> MSEVFLELGQRPDEAGPPISGPATYPDDVTESLRADAEQIIARYPDARSA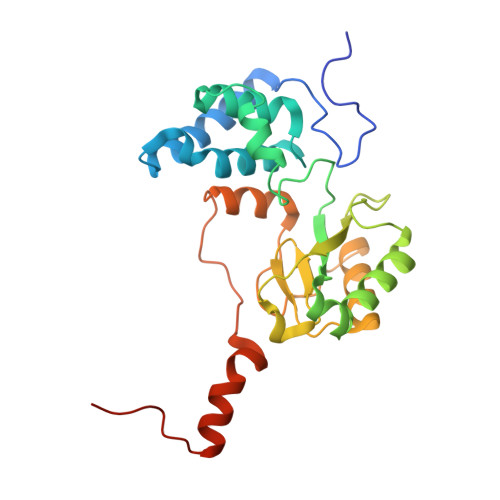LLPLLHLVQAQDGYLTPAGIGFCAAQLGLTEAEVTAVATFYSMYRRTPTGDYLVGVCTNTLCAIMGGDAILEALEDHLGVHPGQTTPDGRVTLEHVECNAACDYAPVVMVNWEFYDNQTPSSARDLVDGLRSGSPPPPTRGSLCTFRETARTLAGLTDPNAPGGAPGAATLAGLRLARERGMTAPTPPQTNGSAS>SGFVCNTCPEKWINFQRKCYYFGKGTKQWVHARYACDDMEGQLVSIHSPEEQDFLTKHASHTGSWIGLRNLDLKGEFIWVDGSHVDYSNWAPGEPTSRSQGEDCVMMRGSGRWNAAFCDRKLGAWVCDRLATCTPPASEGSAE[7x]

The second principal receptor for IgE, CD23, is a type II transmembrane glycoprotein with a C-type lectin-like domain (CTLD)4 (3, 4). In its membrane-bound form, CD23 consists of three CTLD “heads” connected to the membrane via a trimeric α-helical coiled-coil “stalk”. The interaction between CD23 and IgE is critical in the regulation of IgE synthesis, which can be up- or down-regulated depending on the oligomerization state of CD23 (2, 9, 10). We have determined the crystal structures of the human lectin-like head domain of CD23 in its Ca2+-free and Ca2+-bound forms, as well as the crystal structure of the Ca2+-bound head domain of CD23 in complex with a subfragment of IgE-Fc consisting of the dimer of Cϵ3 and Cϵ4 domains (Fcϵ3-4).

To verify that the principal site is indeed the location of Ca2+ binding to derCD23 in solution, and to confirm the exact nature of the interaction, several single point mutations in derCD23 were generated: conserved residues were mutated within the principal (E249A and D270A) and auxiliary (S252A and D258A) calcium-binding sites, along with the highly conserved Asn-269 residue (N269A and N269D). As expected, the two principal binding site derCD23 mutants, E249A and D270A, were unable to bind Ca2+. D258A (auxiliary) and D270A (principal site) crystallized differently, and in all eight and seven molecules within the asymmetric unit, respectively, Pro-250 is trans. The crystal structures of the derCD23 principal and auxiliary Ca2+-binding site mutants were determined (but not those of N269A or N269D mutants). No major conformational changes were observed in either the principal or auxiliary Ca2+-binding sites upon introduction of the point mutations that could inadvertently affect the binding of Ca2+, with the exception of D258A.>[2x]LTLGLAPALSTHSSGVSTQSVDLSQIKRGDEIQAHCLTPAETEVTECAGILKDVLSKNLHELQGLCNVKNKMGVPWVSVEELGQEIITGRLPFPSVGGT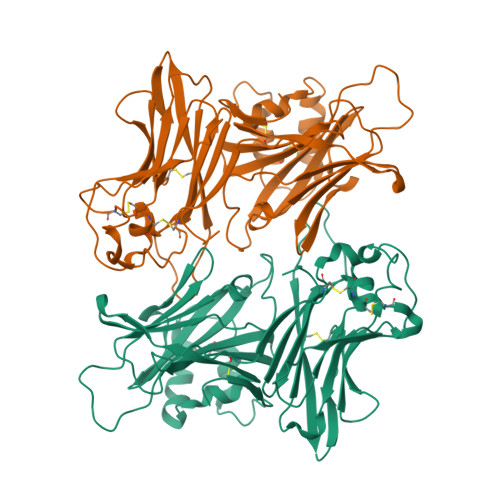PVNDLVRVLVVAESNTPEETPEEEFYAYVELQTELYTFGLSDDNVVFTSDYMTVWMIDIPKSYVDVGMLTRATFLEQWPGAKVTVMIPYSSTFTWCGELGAISEESAPQPSLSARSPVCKNSARYSTSKFCEVDGCTAETGMEKMSLLTPFGGPPQQAKMNTCPCYYKYSVSPLPAMDHLILADLAGLDSLTSPVYVMAAYFDSTHENPVRPSSKLYHCALQMTSHDGVWTSTSSEQCPIRLVEGQSQNVLQVRVAPTSMPNLVGVSLMLEGQQYRLEYFGDH>SMASDMEEKFREAFILFSSCSDHIEMYKFFELMNSFGIILTNDEKAALPNDINMDYWLNFAKKHYNYEQPFKHIN[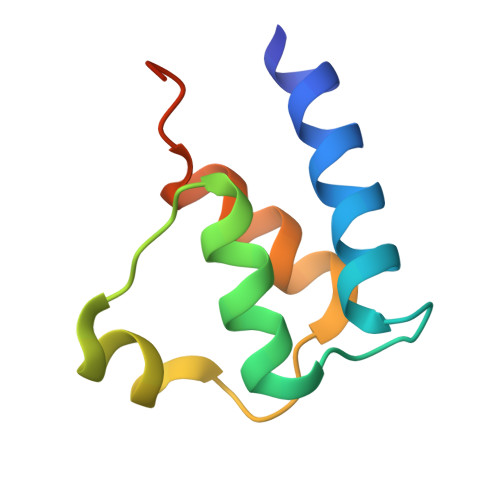2x]4-[4-[(4,4-dimethylpiperidin-1-yl)methyl]phenyl]-1-methyl-9-[6-(methylamino)pyrimidin-4-yl]-1,4,9-triazaspiro[5.5]undecan-2-one | C28 H41 N7 O | 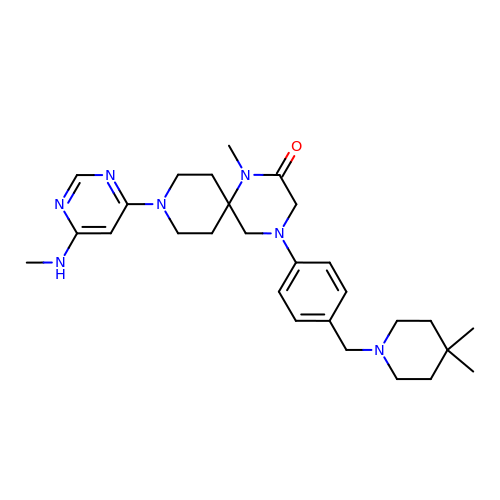QIXCWPPRGHCUNI-UHFFFAOYSA-N> MGMGYQPPSDYKQCKHLKSFPVSELKGDNKELWLMKVPANIDISQLKSLPLDTDATVSTVELGSKNFNVLQNTSTQEGSDNTNLSLLIPSEKKKETLKVATSKDNKSVYFDR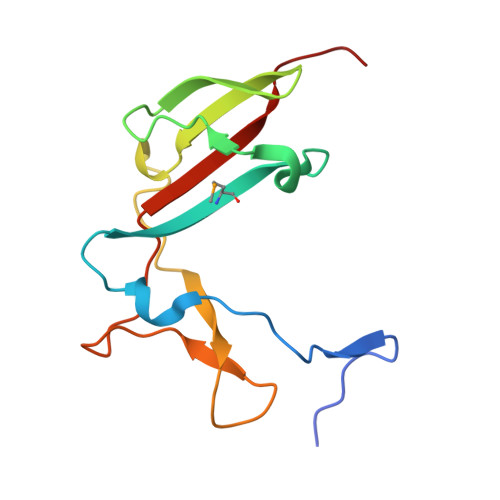VFTISETARIP>SDPKLTKAVDSICDQFIVTKSKISQLTEYFIDCMEKGLEPCENKGLPMIPTFVTDKPSGQEHGVTMLAADLGGTNFRVCSVELLGNHEFKIEQEKSKIPTFFFQDDHHVTSKDLFQHMALITHQFLTKHHKDVIQDYKWKMGFTFSYPVDQTSLSSGKLIRWTKGFKIGDTVGQDVVQLFQQELNDIGLSNVHVVALTNDTTGTLLARCYASSDAARAINEPVIGCIFGTGTNGCYMEKLENIHKLDPASREELLSQGKTHMCINTEWGSFDNELNHLPTTSYDIKIDQQFSTNPGFHLFEKRVSGLYLGEILRNILLDLEKQELFDLKESVLKNNPFILTTETLSHIEIDTVENDLQDTRDALLKAADLETTFEERVLIQKLVRAISRRAAFLAAVPIAAILIKTNALNQSYHCQVEVGCDGSVVEHYPGFRSMMRHALALSPIGPEGERDVHLRISKDGSGVGAALCALHANY[3x]

Glucose-dependent regulation requires glucose phosphorylation provided by glucose-phosphorylating enzymes, glucokinases, and hexokinases. These enzymes are responsible for intracellular trapping and metabolism initiation of monosaccharides and catalyze ATP-driven phosphorylation, yielding ADP and glucose-6-phosphate. The KlGlk1 mutants denoted the role of the enzyme as an accessory glucose phosphorylating protein (to KlHxk1) which might act as a glucose phosphorylation enzyme with currently unknown physiological function. Our study expands the understanding of glucose metabolizing enzymes in K. lactis by presenting the first crystal structure of its unique glucokinase.

We crystallized KlGlk1 in an apo form. The asymmetric unit contains three KlGlk1 molecules and the unit cell belongs to C 2 2 21 space group. KlGlk1 consists of two ribonuclease H-like type domains. The N-terminal, smaller domain K represents compact fold with beta strands in the domain’s core and short alpha helices located between strands 1–3 and 10–13 as well as at the top of domain K (helices 3 and 4). Larger domain Z consists of central mixed β-sheet (strands 10–13) flanked by alpha helices connected by the extended loops resulting in the elongated shape of the domain. Inspection of the overlap among the molecules contained in the asymmetric unit (ASU) does not indicate any significant structural differences as confirmed by low root mean square deviation (RMSD) values calculated by TM-align (RMSD calculated based on backbone C alpha atoms; RMSD values of backbone atoms of chains A/B, B/C and A/C are 0.53 for 469 residues, 0.62 for 469 residues, 0.54 for 470 residues, respectively). Nonetheless, this analysis of the arrangement of molecules in the crystal does not indicate stable dimerization—the buried surface areas are too small to ensure stable dimerization in solution. In KlHxk1, the substrate binding promotes the closed conformation of protein, whereas apo KlGlk1 remains in open state. Moreover, the protein part undergoing conformational change encompasses the region of 115–195 residues that folds into helices H3 and H4 and stands S4–S7 with a 165–174 loop that might be responsible for stabilizing the substrate at the active site of the enzyme. The protein remains inactive when the ATP level in the cell is high, which suggests that KlGlk1 serves as a safety mechanism preventing too fast energy production. Both kinetic analysis and light scattering studies show that KlGlk1 forms a dimer in solution, which is likely related to activity regulation by ATP.> DNMDIDKVDELMQDIADQQELAEEISTAISKPVGFGEEFDEDELMAELEELEQEELDKNLLEISGPETVPLPNVPSIALPSKPAKKKE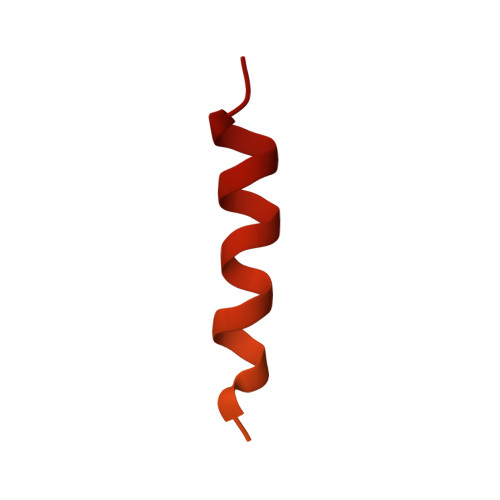EEDDDMKELENWAGSM3-METHYL-4-(THIOPHEN-2-YL)-1H-PYRAZOL-5-AMINE 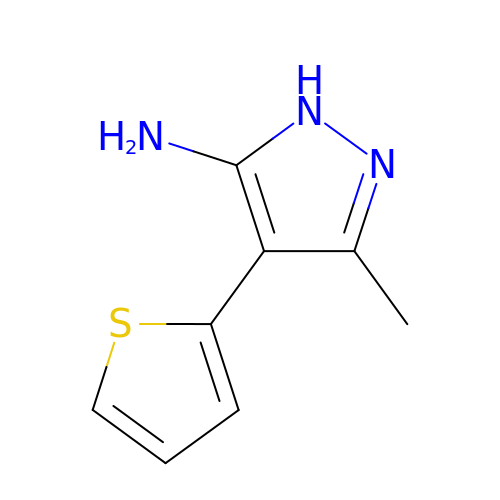| C8 H9 N3 S | LTNSHOVGLDMJRU-UHFFFAOYSA-N>MEFFGESWKKHLSGEFGKPYFIKLMGFVAEERKHYTVYPPPHQVFTWTQMCDIKDVKVVILGQDPYHGPNQAHGLCFSVQRPVPPPPSLENIYKELSTDIEDFVHPGHGDLSGWAKQGVLLLNAVLTVRAHQANSHKERGWEQFTDAVVSWLNQNSNGLVFLLWGSYAQKKGSAIDRKRHHVLQTAHPSPLSVYRGFFGCRHFSKTNELLQKSGKKPIDWKELLEHHHHHH[2x];>MTLELQLKHYITNLFNLPKDEKWECESIEEIADDILPDQYVRLGALSNKILQTYTYYSDTLHES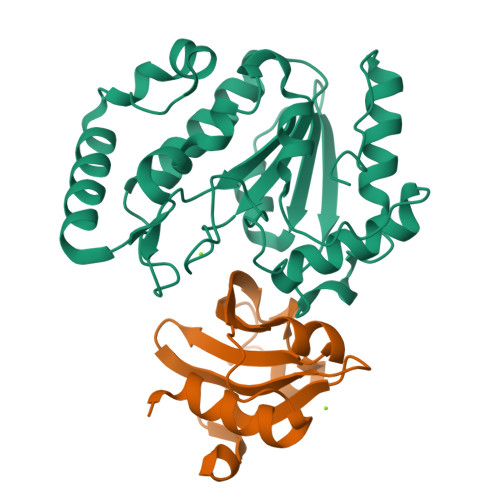NIYPFILYYQKQLIAIGYIDENHDMDFLYLHNTIMPLLDQRYLLTGGQ[2x]> MRGSHHHHHHGSM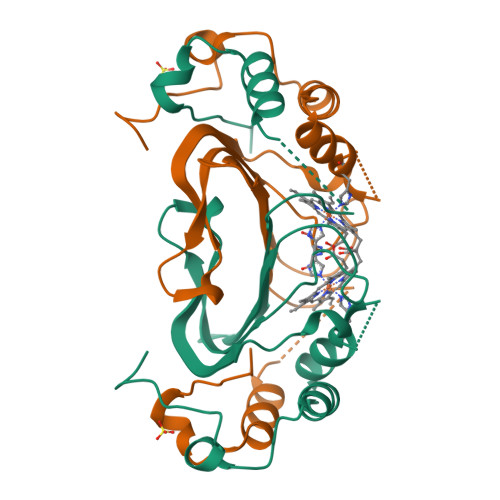STTIQYNSNYADYSISSYLREWANNFGDIDQAPAETKDRGSFSGSSTLFSGTQYAIGSSHSNPEGMIAEGDLKASFMPQHTFHGQIDTLQFGKDLATNAGGPSAGKHLEKIDITFNELDLSGEFDSGKSMTENHQGDMHKSVRGLMKGNPDPMLEVMKAKGINVDTAFKDLSIASQYPDSGYMSDAPMVDTVGVMDSNDMLLAA>MDAPEEEDHVLVLRKSNFAEALAAHKYLLVEFYAPWCGHCKALAPEYAKAAGKLKAEGSEIRLAKVDATEESDLAQQYGVRGYPTIKFFRNGDTASPKEYTAGREADDIVNWLKKRTGPAATTLPDGAAAESLVESSEVAVIGFFKDVESDSAKQFLQAAEAIDDIPFGITSNSDVFSKYQLDKDGVVLFKKFDEGRNNFEGEVTKENLLDFIKHNQLPLVIEFTEQTAPKIFGGEIKTHILLFLPKSVSDYDGKLSNFKTAAESFKGKILFIFIDSDHTDNQRILEFFGLKKEECPAVRLITLEEEMTKYKPESEELTAERITEFCHRFLEGKIKPHLMSQELPEDWDKQPVKVLVGKNFEDVAFDEKKNVFVEFYAPWCGHCKQLAPIWDKLGETYKDHENIVIAKMDSTANEVEAVKVHSFPTLKFFPASADRTVIDYNGERTLDGFKKFLESGGQDGAGDDDDLEDLEEAEEPDMEEDDDQKAVKDEL[2x];>[2x]MHHHHHHMVKGHTTGLSLNNDRLYKLTYSTEVLLDRGKGKLQDSVGYRISSNVDVALLWRNPDGDDDQLIQITMKDVNVENVNQQRGE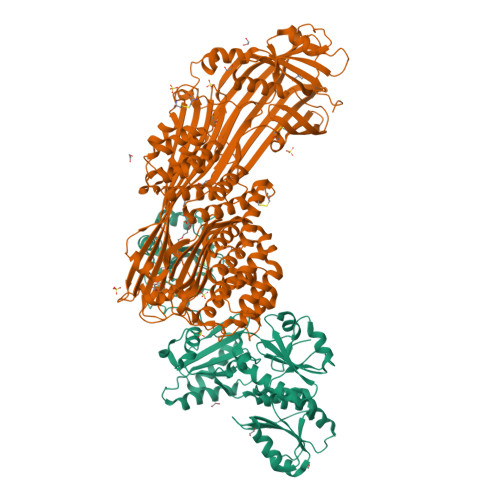KSIFKGKSPSKIMGKENLEALQRPTLLHLIHGKVKEFYSYQNEAVAIENIKRGLASLFQTQLSSGTTNEVDISGNCKVTYQAHQDKVIKIKALDSCKIARSGFTTPNQVLGVSSKATSVTTYKIEDSFVIAVLAEETHNFGLNFLQTIKGKIVSKQKLELKTTEAGPRLMSGKQAAAIIKAVDSKYTAIPIVGQVFQSHCKGCPSLSELWRSTRKYLQPDNLSKAEAVRNFLAFIQHLRTAKKEEILQILKMENKEVLPQLVDAVTSAQTSDSLEAILDFLDFKSDSSIILQERFLYACGFASHPNEELLRALISKFKGSIGSSDIRETVMIITGTLVRKLCQNEGCKLKAVVEAKKLILGGLEKAEKKEDTRMYLLALKNALLPEGIPSLLKYAEAGEGPISHLATTALQRYDLPFITDEVKKTLNRIYHQNRKVHEKTVRTAAAAIILNNNPSYMDVKNILLSIGELPQEMNKYMLAIVQDILRFEMPASKIVRRVLKEMVAHNYDRFSRSGSSSAYTGYIERSPRSASTYSLDILYSGSGILRRSNLNIFQYIGKAGLHGSQVVIEAQGLEALIAATPDEGEENLDSYAGMSAILFDVQLRPVTFFNGYSDLMSKMLSASGDPISVVKGLILLIDHSQELQLQSGLKANIEVQGGLAIDISGAMEFSLWYRESKTRVKNRVTVVITTDITVDSSFVKAGLETSTETEAGLEFISTVQFSQYPFLVCMQMDKDEAPFRQFEKKYERLSTGRGYVSQKRKESVLAGCEFPLHQENSEMCKVVFAPQPDSTSSGWF>[2x]APQALRENILFGMGNPLLDISAVVDKDFLDKYSLKPNDQILAEDKHKELFDELVKKFKVEYHAGGSTQNSIKVAQWMIQQPHKAATFFGCIGIDKFGEILKRKAAEAHVDAHYYEQNEQPTGTCAACITGDNRSLIANLAA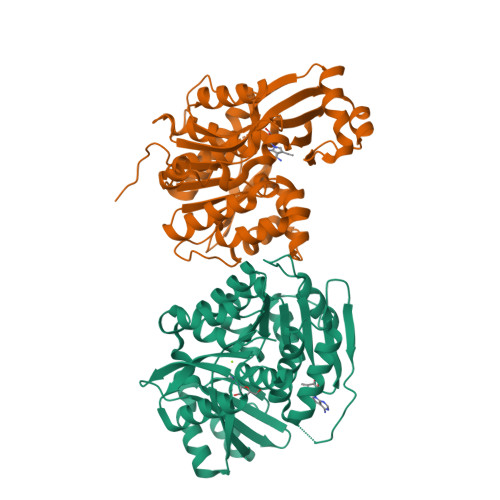ANCYKKEKHLDLEKNWMLVEKARVCYIAGFFLTVSPESVLKVAHHASENNRIFTLNLSAPFISQFYKESLMKVMPYVDILFGNETEAATFAREQGFETKDIKEIAKKTQALPKMNSKRQRIVIFTQGRDDTIMATESEVTAFAVLDQDQKEIIDTNGAGDAFVGGFLSQLVSDKPLTECIRAGHYAASIIIRRTGCTFPEKPDFH Formation of the peptidoglycan stem pentapeptide requires the insertion of both l and d amino acids by the ATP-dependent ligase enzymes MurC, -D, -E, and -F. The stereochemical control of the third position amino acid in the pentapeptide is crucial to maintain the fidelity of later biosynthetic steps contributing to cell morphology, antibiotic resistance, and pathogenesis. The resulting enol-pyruvoyl-UDP-N-acetylglucosamine is reduced with NADPH by MurB, yielding UDP-N-acetylmuramic acid (UDP-MurNAc). This intermediate is then subjected to ATP-dependent aminoacylation with, in sequence, l-alanine, d-glutamate, and either l-lysine or meso-diaminopimelic acid (mDAP), by the sequential action of Mur ligases C, D, and E to produce UDP-MurNAc-tripeptide. As seen with other enzymes of this class, MurESa is composed of a three-domain, mixed α/β structure. Domain 1 extends from residues 1 to 98 encompassing the uridine nucleoside-binding site of the UDP-MurNAc-tripeptide product, domain 2 extends from residues 99 to 332 and encompasses most of the rest of the UDP-MurNAc-tripeptide-binding pocket, and finally, domain 3 extends from residues 333 to 493, with the ATP-binding site formed between domains 2 and 3.

Here we determined the x-ray crystal structure of Staphylococcus aureus MurE UDP-N-acetylmuramoyl-l-alanyl-d-glutamate:meso-2,6-diaminopimelate ligase (MurE) (E.C. 6.3.2.7) at 1.8 Å resolution in the presence of ADP and the reaction product, UDP-MurNAc-l-Ala-γ-d-Glu-l-Lys. This structure provides for the first time a molecular understanding of how this Gram-positive enzyme discriminates between l-lysine and d,l-diaminopimelic acid, the predominant amino acid that replaces l-lysine in Gram-negative peptidoglycan. The structure reveals the enzyme in a ternary product complex with ADP and UDP-MurNAc-l-Ala-γ-d-Glu-l-Lys within the active site in a closed conformation. Although the two structures in this study do not differ substantially, as assessed by comparison of r.m.s.d. values between them, inspection of the ATP-binding site of the product co-crystallization complex shows that two side chains take on a different conformation. These side chains, Phe-300 and Lys-360, are both in the vicinity of the binding site for the adenine ring of ATP. In the case of Phe-300, the phenyl ring is rotated by roughly 90° to accommodate the adenine ring, and this movement displaces a network of two ordered water molecules. As with the E. coli and M. tuberculosis MurE structures, as well as those of the preceding enzyme in the pathway MurD, a specific lysine residue (Lys-219) is post-translationally modified to N-carboxylated lysine within the active site region and is thought to be required for positioning of the Mg2+-ATP complex. In MurESa, the l-lysine residue at position three of the UDP-MurNAc-tripeptide ligand is bound by a relatively small number of electrostatic interactions with the protein.

> MDASTLFKKVKVKRVLGSLEQQIDDITTDSRTAREGSIFVASVGYTVDSHKFCQNVADQGCKLVVVNKEQSLPANVTQVVVPDTLRVASILAHTLYDYPSHQLVTFGVTGTNGKTSIATMIHLIQRKLQKNSAYLGTNGFQINETKTKGANTTPETVSLTKKIKEAVDAGAESMTLEVSSHGLVLGRLRGVEFDVAIFSNLTQDHLDFHGTMEAYGHAKSLLFSQLGEDLSKEKYVVLNNDDSFSEYLRTVTPYEVFSYGIDEEAQFMAKNIQESLQGVSFDFVTPFGTYPVKSPYVGKFNISNIMAAMIAVWSKGTSLETIIKAVENLEPVEGRLEVLDPSLPIDLIIDYAHTADGMNKLIDAVQPFVKQKLIFLVGMAGERDLTKTPEMGRVACRADYVIFTPDNPANDDPKMLTAELAKGATHQNYIEFDDRAEGIKHAIDIAEPGDTVVLASKGREPYQIMPGHIKVPHRDDLIGLEAAYKKFGGGPVDRSHHHHHH> MIAAQLLAYYFTELKDDQVKKIDKYLYAMRLSDETLIDIMTRFRKEMKNGLSRDFNPTATVKMLPTFVRSIPDGSEKGDFIALDLGGSSFRILRVQVNHEKNQNVHMESEVYDTPENIVHGSGSQLFDHVAECLGDFMEKRKIKDKKLPVGFTFSFPCQQSK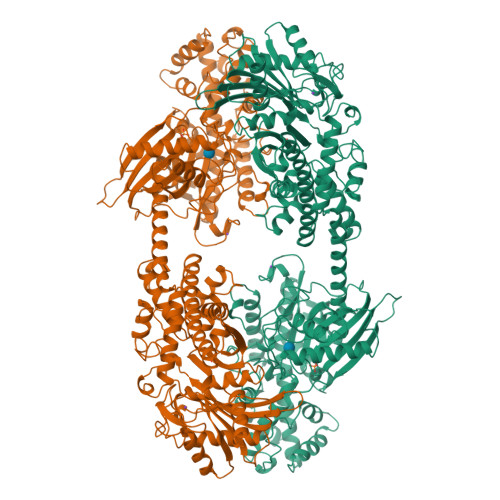IDEAILITWTKRFKASGVEGADVVKLLNKAIKKRGDYDANIVAVVNDTVGTMMTCGYDDQHCEVGLIIGTGTNACYMEELRHIDLVEGDEGRMCINTEWGAFGDDGSLEDIRTEFDREIDRGSLNPGKQLFEKMVSGMYLGELVRLILVKMAKEGLLFEGRITPELLTRGKFNTSDVSAIEKNKEGLHNAKEILTRLGVEPSDDDCVSVQHVCTIVSFRSANLVAATLGAILNRLRDNKGTPRLRTTVGVDGSLYKTHPQYSRRFHKTLRRLVPDSDVRFLLSESGSGKGAAMVTAVAYRLAEQHRQIEETLAHFHLTKDMLLEVKKRMRAEMELGLRKQTHNNAVVKMLPSFVRRTPDGTENGDFLALDLGGTNFRVLLVKIRSGKKRTVEMHNKIYAIPIEIMQGTGEELFDHIVSCISDFLDYMGIKGPRMPLGFTFSFPCQQTSLDAGILITWTKGFKATDCVGHDVVTLLRDAIKRREEFDLDVVAVVNDTVGTMMTCAYEEPTCEVGLIVGTGSNACYMEEMKNVEMVEGDQGQMCINMEWGAFGDNGCLDDIRTHYDRLVNEYSLNAGKQRYEKMISGMYLGEIVRNILIDFTKKGFLFRGQISETLKTRGIFETKFLSQIESDRLALLQVRAILQQLGLNSTCDDSILVKTVCGVVSRRAAQLCGAGMAAVVDKIRENRGLDRLNVTVGVDGTLYKLHPHFSRIMHQTVKELSPKCNVSFLLSEDGSGKGAALITAVGVRLRTEASS>SNAMSKLPENFLWGGAVAAHQLEGGWQEGGKGISVADVMTAGRHGVAREITAGVLEGKYYPNHEAIDFYHHYKEDVKLFAEMGFKCFRTSIAWTRIFPKGDEAEPNEAGLQFYDDLFDECLKYGIEPVVTLSHFELPYHLVTEYGGFTNRKVIDFFVHFAEVCFRRYKDKVKYWMTFNEINNQANYQEDFAPFTNSGIVYKEGDDREAIMYQAAHYELVASARAVKIGHAINPNLNIGCMVAMCPIYPATCNPKDILMAQKAMQKRYYFADVHVHGFYPEHIFKYWERKAIKVDFTERDKKDLFEGTVDYIGFSYYMSFVIDAHRENNPYYDYLETEDLVKNPYVKASDWDWQIDPQGLRYALNWFTDMYHLPLFIVENGFGAIDQVEADGMVHDDYRIDYLGAHIKEMIKAVDEDGVELMG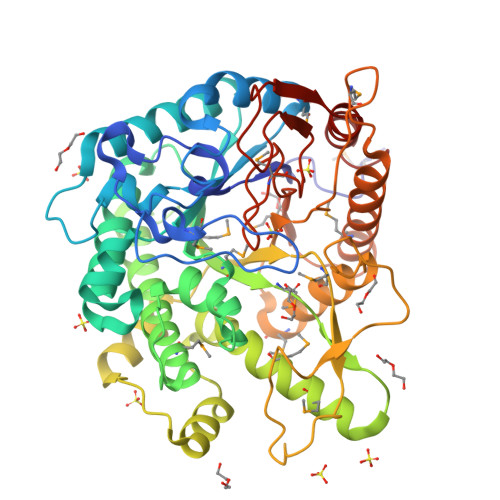YTPWGCIDLVSAGTGEMRKRYGFIYVDKDDEGKGTLKRSPKLSFNWYKEVIASNGDDI[2x]> MSEFRIHHDVNELLSLLRVHGGDGAEVYIDLLQKNRTPYVTTTVSAHSAKVKIAEFSRTPEDFLKKYDELKSKNTRNLDPLVYLLSKLMEDRETLQYLQQNAKERAELAASAAASSTASFGASATASKISMQELEELRKQLGSVATGPTWQQSLELTRKMLRDKQSKKNSGQRLPVLPAWVYERPALLGDFLPGTGGSADTAVPIGSLPLASQEAAVVEDLLYVLVGVDGRYISAQPLTGRQGRTFLVDPNLDLSIRELVSRILPVAASYSTVTRFIEEKSSFEYGQVNHALAAAMRTLVKEYLVLVTQLEQLQRQGLLSLQKLWFYIQPAMRSLDILASLATSVDKGECIGGATLSLLHDRSFSYTGDSQAQELCLHLTKAASTPYFEILEKWIYRGIIDDPYSEFMVEEHELRKEKIQEDYNDKYWDQRYTVVQRQIPSFLQKMAGKVLSTGKYLNVVRECGHDVTCPVAKEVVYTLKERAYVEQIEKAFSYASKVLLDFLM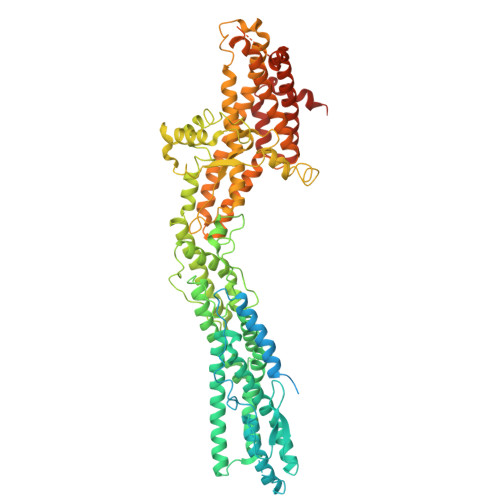GEKELLAHLRSIKRYFLMDQGDFFVHFMDLTEEELKKPVDDITPTRLEALLELALRMSTANTDPFKDDLKIDLMPHDLITQLLRVLAIETQQEKAMVHADPTELTLSGLEAFSFDYVVTWPLSLIINRKALTRYQMLFRHMFYCKHVERQLCSVWISNKAAKRFSLHSAKWFAGAFTLRQRMLNFVQNIQSYMMFEVMEPTWHVLEQNLRSASNIDDVLGHHASFLDNCLKDCMLTNPELLRVFSKLMSVCVMFTNCLQRFTQSMKLDSELGHPALEPGAMLGPPTEAERAEERARKELARKCLAEHVDAPQLASSFEATITKFDKNFSAHLLDLLARLSIYSTSDCEHGMASVISRLDFNGFYTERLERLSAERSQKAAPPVPGPRGPPALVPRVAVTAQ> MGSSKPLKGFVICCTSIDLKQRTEISTKATKLGAAYRSDFTKDVTHLIAGDFDTPKYKFAAKSRPDIKIMSSEWIPVLYESWVQGEDLDDGLLVDKHLLPTLFKCRVCLTNIGQPERSRIENYVLKHGGTFCPDLTRDVTHLIAGTSSGRKYEYALKWKINVVCVEWLWQSIQRNAVLEPQYFQLD;> GYDSILVQATPRKSSSVITELPDTPIKMNS

TOPBP1 and its fission and budding yeast orthologues Rad4 and Dpb11, respectively, are scaffold proteins that mediate formation of multi-protein complexes in a range of essential DNA replication and repair processes. Bioinformatic analysis suggests that only three of the BRCT domains in the yeast TOPBP1 homologues, and four in the vertebrate TOPBP1 homologues, possess the required cluster of residues needed to bind phosphorylated peptide motifs. Despite the structural similarity of these phosphopeptide-binding BRCT domains, genetic and biochemical studies show that they are nonetheless selective and specific for the phosphopeptide sequences with which they interact. To gain some insight into this, we have determined crystal structures of segments of yeast and vertebrate TOPBP1 that contain the two most N-terminal phosphopeptide binding sites (BRCT1 and BRCT2), in complex with phosphopeptides derived from a number of different known ligand proteins, including RAD9, and used this to develop consensus patterns that encapsulate the individual specificity requirements of these two independent binding sites.

We have now also determined the crystal structure of a bis-phosphorylated pT636-pT650 peptide from Sld3 (the fission yeast homologue of Treslin), which interacts simultaneously with Rad4-BRCT1 and Rad4-BRCT2, albeit with different molecules in the asymmetric unit of the crystals. In these complexes, the peptide backbone upstream of the phosphorylated residue maintains a consistent β-sheet conformation, and does not contain the tight turn seen for the hydrophobic triplets in peptides bound to the BRCT1 domain of TOPBP1 or Rad4. In BRCT2, however, the size of the recess is restricted by the side chain of a highly conserved tryptophan residue (Trp158 in Rad4; Trp257 in human TOPBP1) at the C-terminal end of the α-helix, and can only accommodate a single hydrophobic side chain, requiring that the peptide chain continues in an extended β-sheet conformation. Sequences with hydrophobic residues at −3 and −4 (and often −5) as in the RAD9-pS387, Crb2-pT187, Sld3-pT636 and Treslin-pS1001 (993-DIGVVEEpSP) peptides conform to this requirement, whereas sequences with large polar side chains such as Crb2-pT235 where −4 is arginine, or Sld3-pT650 where −4 is glutamate, do not, and are restricted to binding to BRCT2.> MGNMERDLFEKKFKEIKDKWVTDKQADEFIETADKYADKA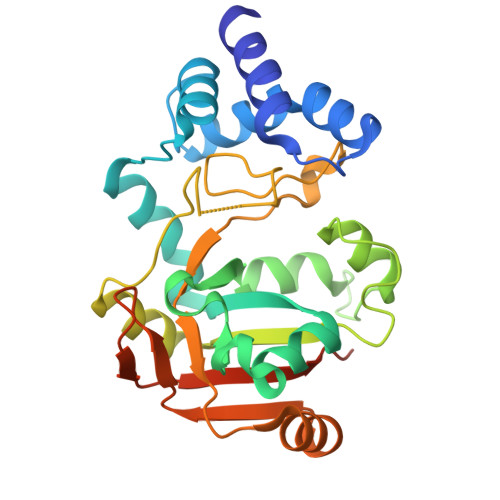VQMSAVASRAEYYRMYVSRKYHYKKEFVEKLKQVYKESGASHVTSKKDLMLAFDDAKRKSTIGRQENGLFVTSFAEDMALLFTDQGKLKSADQIENIKDVDSGKYSDGVYQYEYDSELTKNIDKLGYIRTASGDTPRANSLNIPGCQTWSGKHIENSESELIFPSISVKDLKSKAVLAEIDAKGYFEIIDPTIIAPNGDHKKVTGRFKIKKMQDRMQDRKLEHHHHHH>MGVHTFEEESTSPVPPAKLFKATVVDGDELTPKLIPAIQSIEIVEGNGGPGTVKKVTAVEDGKTSYVLHKIDAIDEATYTYDYTISGGTGFQEILEKVSFKTKLEAADGGSKIKVSVTFHTKGDAPLPDEVHQDVKQKSQGIFKAIEGYVLSN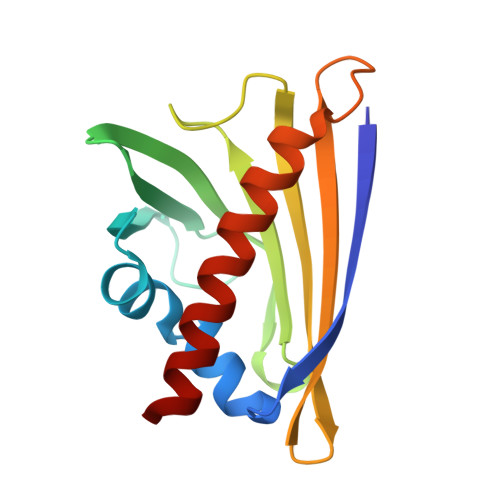[8x]> MKPYVLKFQEIRPHSEALVGGKGMNLGACSNIEGVHVPAGFCLTTEAYKRTLAENNEFTQLLQRLSSLKTSDMDAIREISETIRTLIQHTQIPSEIASYMDATLLDVGGYEMPFAVRSSATAEDLPHASFAGQHDTYLNIIGKDALLQHISMCWASLFTERAIIYRIQNQFDHRKVQLAVVIQQMISPEASGILFTADPITSNRKSLSIDASFGLGEALVSGLVSADSYTVRENTITNKIIATKKLAIYSLKEGGTETRILEKSQQTKQTLTDQQIIQLAKLGRKIEAYFGKPQDIEWCLAEGAFYIVQSRPITTLYPIPEVNEPGNRVYISVAHQQMMTDAMKPLGLSFYLMTTPATMYTAGGRLFVDITQSLSAKVSRDMMVNSLGQSDPLIKDA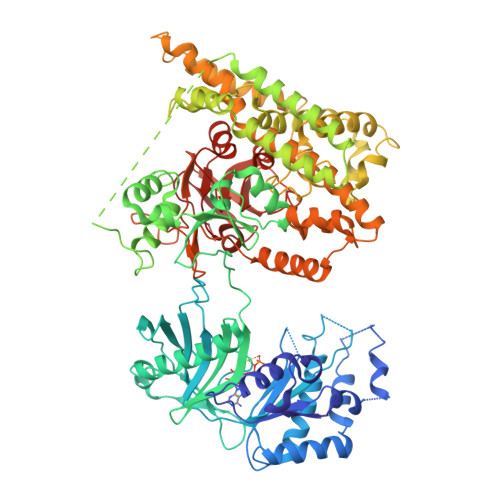LLTVINKKGFLPPLPTEENPSHATVSGKPPVRSIPDSSSVFELVRNSENSIKHLKQSIETKSGSDLFDFIVEDLEELKRVLFNPTSIDAIMAGMDASAWLNEHIYQWLGEKNVADKLSESAPNNITSQMGLELLDVADVIRPYPAVRAYLEQTKNPDFMNELATLEGGAETKKALEDYLQKYGMRCAGEIDLTKTRWIENPLTLIPLILSNIKNFDSSASMHKFAQGEKEAFHKEQEILRRLQELPDGEQKAMETKEKIDILRHFIGYREYPKYGMINRYFIYKLALLRAGEQLVKDGILQEHEDIYFLYFEELREVVRTGQVDYELINARKRDFATFEKLTPPRILTSDGEMINGEYKRENLPKDAILGLPVSSGTVEGRARVILEMEKADLEDGDILVTAYTDPSWTPAFVSIKGLVTEVGGLMTHGAVIAREYGLPAVVGVENATTIIKDGQQIRINGTEGYIEILD>EAPYASLTEIEHLVQSVCKSYRETCQLRLEDLLRQRSNIFSREEVTGYQRKSMWEMWERCAHHLTEAIQYVVEFAKRLSGFMELCQNDQIVLLKAGAMEVVLVRMCRAYNADNRTVFFEGKYGGMELFRALGCSELISSIFDFSHSLSALHFSEDEIALYTALVLINAHRPGLQEKRKV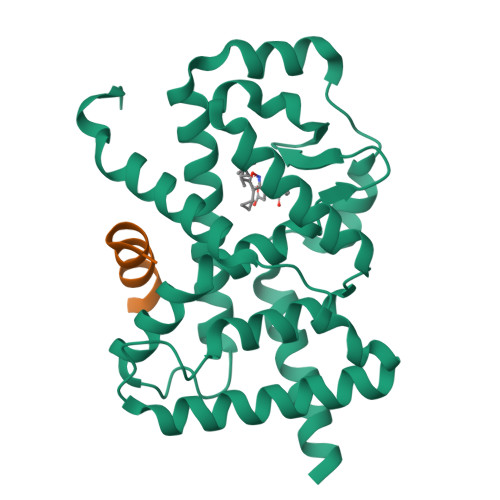EQLQYNLELAFHHHLCKTHRQSILAKLPPAGKLASLCSQHVERLQIFQHLHPIVVQAAFPPLYKELFSTETESPVGLSK[4x];>[4x]TNMGLEAIIRKALMGKYDQWEE> MSLRRGIYHIENAGVPSAIDLKDGSSSDGTPIVGWQFTPDTINWHQLWLAEPIPNVADTFTLCNLFSGTYMDLYNGSSEAGTAVNGWQGTAFTTNPHQLWTIKKSSDGTSYKIQNYGSK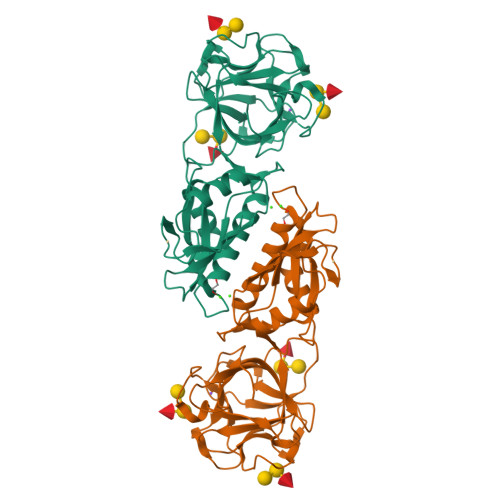TFVDLVNGDSSDGAKIAGWTGTWDEGNPHQKWYFNRMSVSSAEAQAAIARNPHIHGTYRGYILDGEYLVLPNATFTQIWKDSGLPGSKWREQIYDCDDFAIAMKAAVGKWGADSWKANGFAIFCGVMLGVNKAGDAAHAYNFTLTKDHADIVFFEPQNGGYLNDIGYDSYMAFY> DYKDDDDLEVLFQGPGGSSAPARPNWLAYDWGLVFLVAAIVALGFVNLGSAAPDPVLLYRQSVALGLGLLLAFLLQFLSRRRLFGLAYPLYGASLLLLALVLVVGREINGARAWFVLGPLQFQPLELAKLGLLLALAKALEGRPIARVWDYALPALLTLPVVGLLLLQPDLGGALVVLFGVFVVVFVRGLPWRHLLVGLFALALLVPTAVWPNLKPYQRERVLIVLDPYRDPLGQGFQVIQSTIAIGSGGLFGKGYGQGTQAQLGFIPFRHTAFVFSVWAEEWGFVGVVGLLGLYGLLLARLFALALACPRLSDRLFLSGFAGMLGFQVVVNLGVALGVMPVTGLTLPLFSYGGSSLIATLAGLGLVLLVHRDRYQD;> MGTGRIHALALFFALALFLLGLRAWQLQVLEYERYALRSQGNYLKTEDIPAPRGKILDRKGRVLAQDRLVVDLVYTGGEVAFKERLLPLLGLEDLPQVTEPTVLKAGVPEALRPTLEELTAGQKNLYLRERIERYYPNPISGPVMGYVLRANAAQVKQGYSPEEEVGQAGLEAALEPYLRGKRGVRAVEVNVRGERLRETVLEEPTPGQDVVLTLDLALQRAAEKALEEALADINAGRRLNGLPEEKQVKGAIVALDPTTGEVLAMASAPSFDPNLFAKRPVPEEAKALLEDKNLPLLNRAVQPYTPGSTFKLATSYALLEEGYVTPATTYRCSPYIVFGGQVRRNWASRDMGPMTVREAIAWSCNTWYYQAVAQDPLGFVDRLARRARLLGLGEATGLEVAEKTGLLPTRAWKREALGEPWYPGETLSVAIGQGAVLATPAQIARMLATIATGGNKPALHLVKAIGGVPVQPRWEKVPGRYWKVLQE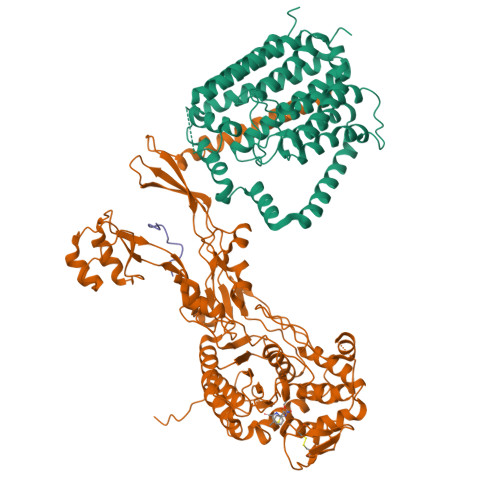GLRKTVSEGTARFVLGEFPVPTGGKTGTAETPGKRRGLEHAWYMGYGPTDGSPYPPLVVVAFFENGGEGSRVALPAVRKVMAAYWGIKGSLEVLFQGPEDQVDPRLIDGK>[4x]MNVEEMKKIAAKEALKFIEDDMVIGLGTGSTTAYFIKLLGEKLKRGEISDIVGVPTSYQAKLLAIEHDIPIASLDQVDAIDVAVDGADEVDP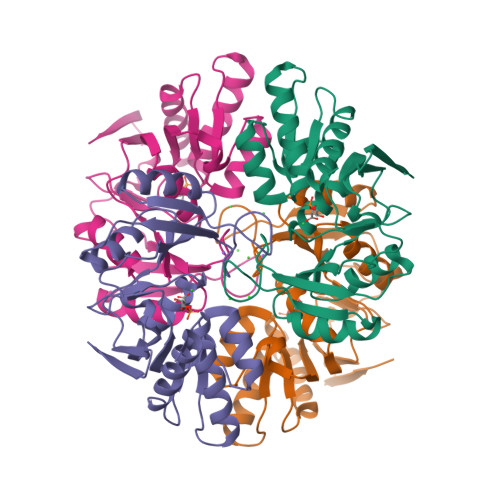NLNLIKGRGAALTMEKIIEYRAGTFIVLVDERKLVDYLCQKMPVPIEVIPQAWKAIIEELSIFNAKAELRMGVNKDGPVITDNGNFIIDAKFPRIDDPLDMEIELNTIPGVIENGIFADIADIVIVGTREGVKKLER> TTGHSYEKYNNWETIEAWTKQVTSENPDLISRTAIGTTFLGNNIYLLKVGKPGPNKPAIFMDCGIHAREWISHAFC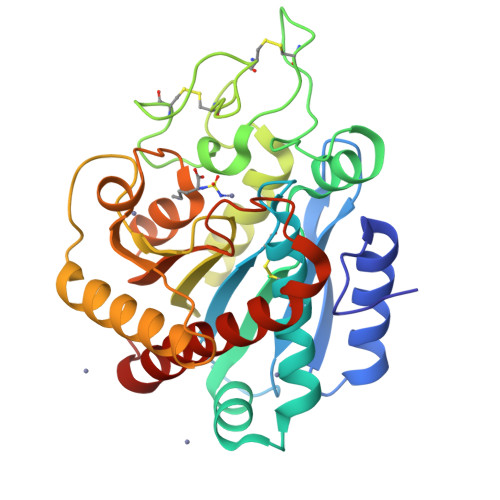QWFVREAVLTYGYESHMTEFLNKLDFYVLPVLNIDGYIYTWTKNRMWRKTRSTNAGTTCIGTDPNRNFDAGWCTTGASTDPCDETYCGSAAESEKETKALADFIRNNLSSIKAYLSIHSYSQHIVYPYSYDYKLPENNAELNNLAKAAVKELATLYGTKYTYGPGATTLYLAPGGGDDWAYDQGIKYSFTFELRDKGRYGFILPESQIQATCEETMLAIKYVTNYVLGHLY>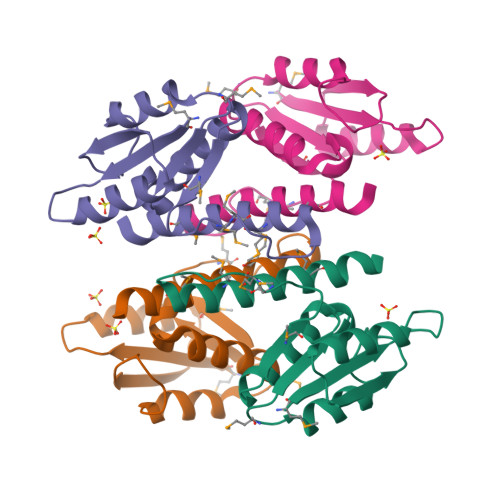[12x]MIIGYARVSSLDQNLERQLENLKTFGAEKIFTEKQSGKSIENRPILQKALNFVEMGDRFIVESIDRLGRNYNEVIHTVNYLKDKEVQLMITSLPMMNEVIGNPLLDKFMKDLVIQILAMVSEQERNES>[4x]MRRHGFSLLELLLASVLMGSLLLVVLALENSSATLRERERARGRLADELSLTATVLARELYTVG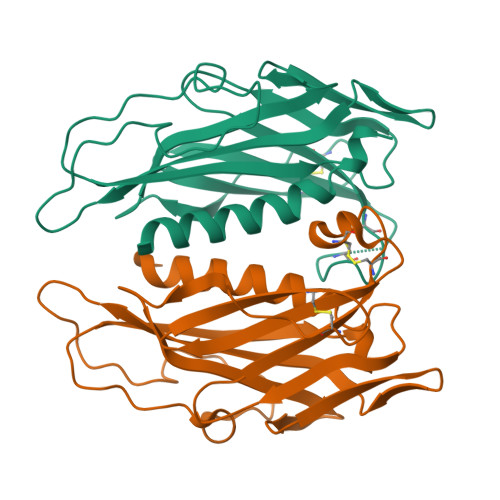YRLTGQALVLSPSSQGDGVQGWFLCEAGMEEICGESMGEVRGTGYEVNQGALRWGACKGEGCAPLPNNPVLGGDEVQVEAFRVAYLEGGTWKRQAQAVNLRPEGASPKVSALALYLLASVPVRGGAPAFTPGSTLSYPPGLTSSLLELPGAPNDGRLRAEKLWIVQTPNLAR> GSGGSGKVVKFSYMWTINNFSFCREEMGEVIKSSTFSSGANDKLKWCLRVNPKGLDEESKDYLSLYLLLVSCPKSEVRAKFKF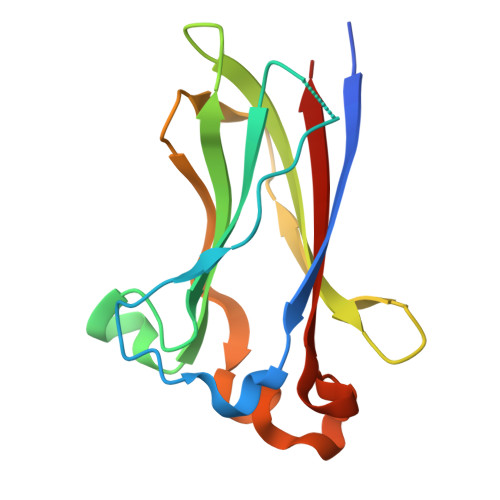SILNAKGEETKAMESQRAYRFVQGKDWGFKKFIRRGFLLDEANGLLPDDKLTLFCEVSVVQD4-formyl-3-hydroxy-8-methoxy-1,9-dimethyl-11-oxo-11H-dibenzo[b,e][1,4]dioxepine-6-carboxylic acid 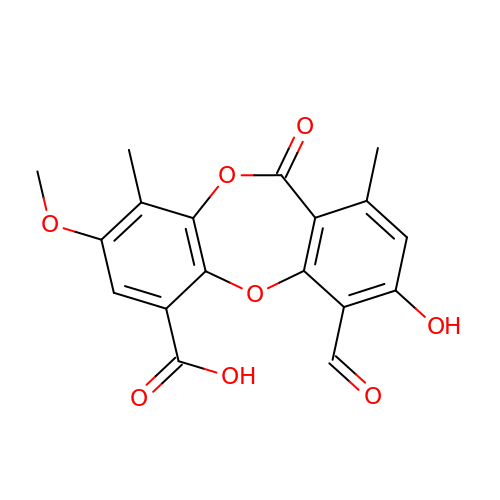| C18 H14 O8 | FUCWJKJZOHOLEO-UHFFFAOYSA-N> MHHHHHHAMAQLGEMVTVLSIDGGGIRG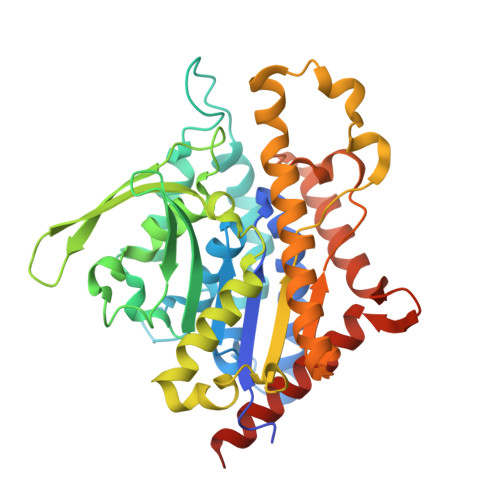IIPATILEFLEGQLQEMDNNADARLADYFDVIGGTSTGGLLTAMISTPNENNRPFAAAKEIVPFYFEHGPQIFNPSGQILGPKYDGKYLMQVLQEKLGETRVHQALTEVVISSFDIKTNKPVIFTKSNLANSPELDAKMYDISYSTAAAPTYFPPHYFVTNTSNGDEYEFNLVDGAVATVADPALLSISVATRLAQKDPAFASIRSLNYKKMLLLSLGTGTTSEFDKTYTAKEAATWTAVHWMLVIQKMTDAASSYMTDYYLSTAFQALDSKNNYLRVQENALTGTTTEMDDASEANMELLVQVGENLLKKPVSEDNPETYEEALKRFAKLLSDRKKLRANKASY> MGSSHHHHHHSSGENLYFQGHMDISEWEKRYNEAYSDISKSLKKVKGIFVAYNSNIDAIKHIDEDDIEKLLEQVDAKEVQERIMEYPRQIDSPADFVARLIISMRDGKAAEVPTYTTDIHEWLTDNLGFDEARMGGQAGIISNLLANMGIKNVIAYVPWLSKEQAEYFVDSENLLHPVVENGKLELKHPKEAYNPDNKPKVNWIIEFSKGLEVKFAGEKIVVPRDNRLIVSSRPPWIRIDMSEELYEHLPEIGKNIDGAILSGYQMIKEEYEDGKTYKDYVEKAVNVIKRLKEGNPDIRIHVEFTSIQNKLIRKAILKDIVRKHVHSLGLDTVEVANALNVLGYEELAYSVIKKDENAIVALYEGAVILLHELKLERVHVHSLGYYICVVSKDSPVSPEDHRKSLLFASTVAAARALLGNINSLDDIEAGLDVPVSEQGYNQLEKLEKYLVRRGICTLEDFENGCICTPNHDVIIIPTKVVEKPVATVGIGDTISAAAFVSVLAKMKKKNE

Nonetheless, in some archaea from the phylum Euryarchaeota, a modified version of this pathway has been described, where glucose and fructose-6-phosphate (F6P) are phosphorylated by homologous enzymes that use ADP instead of ATP as phosphoryl donor. These ADP-dependent sugar kinases can be specific for glucose (ADP-glucokinase [ADP-GK]), fructose-6P (ADP-phosphofructokinase [ADP-PFK]), or bifunctional able to use both substrates (ADP-PFK/GK). The ADP-dependent sugar kinases belong to the ribokinase superfamily and their members display a highly two-domain conserved architecture, a large domain with a Rossmann-like fold and a small α/β domain that acts a lid of the active site. The active site is located in a cleft between both domains, connected by a region of flexible loops that act as a hinge during the ligand-induced conformational change.

Here, we report the crystallographic structure of an ancestral ADP-PFK in ternary complex with F6P and Mg-ADPβS, being the first structure of an enzyme from the ADP-dependent family with F6P at its active site. The structure of the AncMsPFK in complex with F6P-Mg-ADPβS was solved by molecular replacement and refined at 3.12 Å resolution to Rwork/Rfree values of 0.24/0.27. The AncMsPFK crystal contained one molecule per asymmetric unit with 460 of the expected 490 residues, and the unit cell corresponds to P 212121. However, 28 residues from the small domain cannot be solved in this structure; 24 of them belong to helices α2 and α3 and 4 from a β-turn located between β-sheets β9 and β10. Analysis of residues involved in sugar binding shows that F6P is mainly stabilized by hydrogen bond interactions. The strictly conserved D471 residue belongs to the GXGD motif and corresponds to the catalytic base that activates the hydroxyl group of the sugar to be phosphorylated, for the nucleophilic attack toward the ADP. The phosphate group makes contacts with N32, N34, E90, N181, K179, and Q244. On the other hand, the Mg-ADPβS complex is located in a shallow pocket in the large domain establishing hydrogen bonds and hydrophobic interactions with protein residues. Despite the relatively low resolution of the structure, four water molecules around the Mg2+ ion were located, assuming its classical octahedral coordination geometry, which is in agreement with the electronic density of that region. Analysis of residues involved in the stabilization of the close conformation of AncMsPFK reveals several interactions between the large and the small domains, governed by hydrogen bonds. These polar interactions include residues located close to F6P (R212-Q244 and E90-T284), and others such as arginine residues, far away from this sugar (R67-Q287 and R112-G397).>[2x]MEKPAEQVHLSGPTMGTTYNIKYIQQPGIADSKTLQTEIDRLLEEVNDQMSTYRKDSELSRFNQHTSSEPFAVSTQTLTVVKEAIRLNGLTEGALDVTVGPLVNLWGFGPEARPDVVPTDEELNARRAI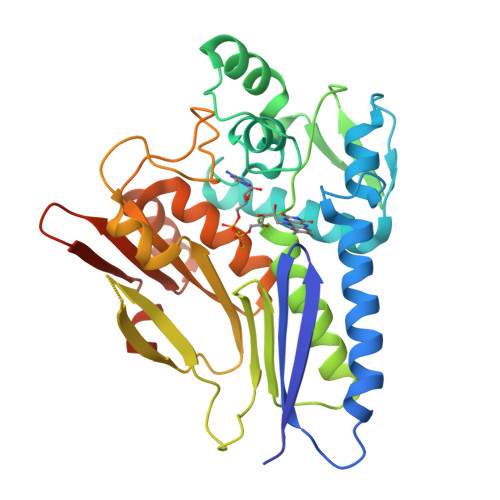TGIEHLTIEGNTLSKDIPELYVDLSTIAKGWGVDVVADYLQSQGIENYMVEIGGEIRLKGLNRDGVPWRIAIEKPSVDQRSVQEIIEPGDYAIATSGDYRNYFEQDGVRYSGIIDPTTGRPINNRVVSVTVLDKSCMTADGLATGLMVMGEERGMAVAEANQIPVLMIVKTDDGFKEYASSSFKPFLSKGGGGHHHHHH6-(CYCLOHEXYLAMINO)-9-[2-(4-METHYLPIPERAZIN-1-YL)-ETHYL]-9H-PURINE-2-CARBONITRILE 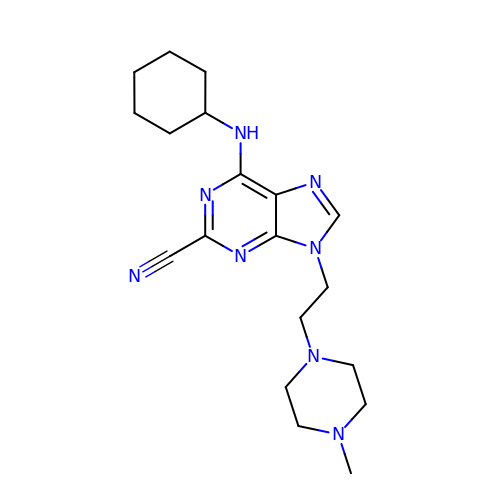| C19 H28 N8 | OGODDSLNRULSMM-UHFFFAOYSA-N>[2x]MSKCLQQLKRQLQHFGIDGCSLADGDIDYFFTVTGIDRGWGCGWRNIQMLISWLQYTNP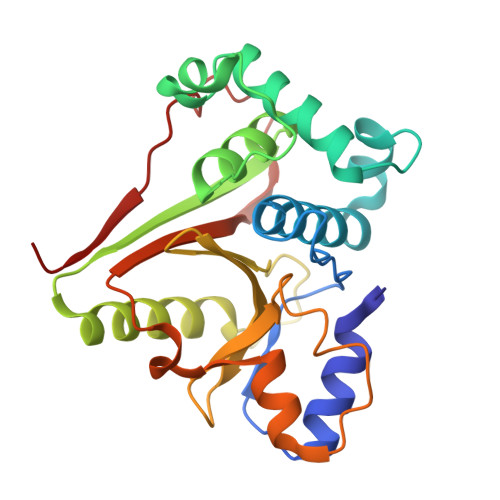NWFKRNFSSGNYEINSLQSLLLSAWMKGIDAEGYAQLGDNLHGKWIGATEVYSLFTGLFVNVALVDFDFRSEASASNALFLYVKKHFESSNDTSNVSPCYLQFQGHSIIIIGFCSSLETLVVLDPDRYQSVQKKFVNIADFNHCYMRKKRSLKFSQFQLVHFKQNIFLNDFSSKLEVRSTRISDF>[4x]MRKIVVAAIAVSLTTVSITASASADPSKD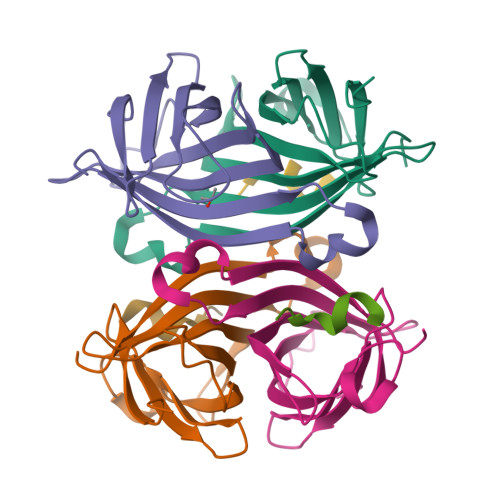SKAQVSAAEAGITGTWYNQLGSTFIVTAGADGALTGTYESAVGNAESRYVLTGRYDSAPATDGSGTALGWTVAWKNNYRNAHSATTWSGQYVGGAEARINTQWLLTSGTTEANAWKSTLVGHDTFTKVKPSAASIDAAKKAGVNNGNPLDAVQQ;>GYGLANVDESSG[3x]>MKEEKRSSTGFLVKQRAFLKLYMITMTEQERLYGLKLLEVLRSEFKEIGFKPNHTEVYRSLHELLDDGILKQIKVKKEGAKLQ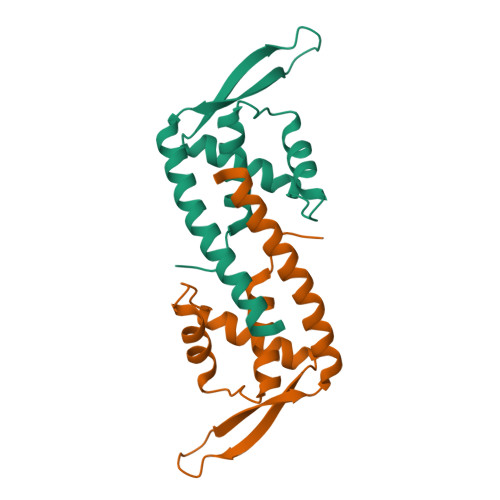EVVLYQFKDYEAAKLYKKQLKVELDRSKKLIEKALSDNF[2x]Langerin, a C-type lectin on Langerhans cells, mediates carbohydrate-dependent uptake of pathogens in the first step of antigen presentation to the adaptive immune system. The extracellular portion of langerin contains a C-type carbohydrate recognition domain (CRD)2 that binds sugars and a neck region that mediates formation of trimers stabilized by a coiled-coil of α-helices. As in other C-type lectins, the CRD of langerin contains a primary Ca2+-dependent sugar-binding site where Ca2+ forms direct coordination bonds with two vicinal hydroxyl groups of a monosaccharide. Langerin binds to a diverse set of glycan ligands including high mannose structures, β-glucans, and fucosylated blood group antigens.

A version of the truncated, trimeric langerin mimicking the naturally occurring minor allele with Asn-288 mutated to aspartate and Lys-313 changed to isoleucine (langerin-D288/I313) was created and compared with the form with only the K313I change (langerin-I313) and wild type langerin. To determine the molecular basis for the enhanced binding of GlcNAc-terminated glycans caused by the K313I change, crystal structures of the carbohydrate recognition domains of langerin-I313, langerin-D288/I313, and wild type langerin in complex with GlcNAc, α-Me-GlcNAc, and two GlcNAc-terminated trisaccharides (GlcNAcβ1-3Galβ1-4Glcβ-CH2CH2N3 (TR54) and GlcNAcβ1-3Galβ1-4GlcNAcβ-CH2CH2N3 (TR55)), representing the terminal portions of poly N-acetyllactosamine chains that are ligands for langerin detected on the glycan array, were solved. Because several of the structures show the same interactions, to simplify presentation of the results, only the data sets that gave the highest resolution structures are shown: wild type langerin CRD bound to α-Me-GlcNAc and trisaccharide TR54, langerin-I313 CRD bound to α-Me-GlcNAc and trisaccharide TR54, and langerin-D288/I313 CRD bound to α-Me-GlcNAc, α-Me-Man and trisaccharide TR55. Structures of the double mutant, with Asp-288 as well as Ile-313, with α-Me-GlcNAc, and with the extended GlcNAc-containing oligosaccharides, showed exactly the same pattern of interactions of the N-acetyl group as were observed for the Ile-313 mutation alone. Thus, the differences in the interactions of Lys-313 and Ile-313 described for the single site mutant can account for the enhanced binding of GlcNAc to the naturally occurring Asp-288/Ile-313 variant as compared with the wild type CRD. However, in all the observed orientations, there are hydrogen bonds between the subterminal galactose residue and the side chain of Lys-299. These contacts would not be affected by the variations at positions 288 or 313. The K313I polymorphism is tightly linked to another SNP that results in the change N288D, which reduces affinity for glycan ligands by destabilizing the Ca2+-binding site.

>[4x]QVVSQGWKYFKGNFYYFSLIPKTWYSAEQFCVSRNSHLTSVTSESEQEFLYKTAGGLIYWIGLTKAGMEGDWSWVDDTPFNKVQSARFWIPGEPNDAGNNEHCGNIKAPSLQAWNDAPCDITFLFICKRPYVPSEP> MRGSHHHHHHENLYFQGSLAVAEPVVNAADAKGTNVNDKVTASDFKLEKTAFDPNQSGNTFMAANFKVTGQVKSGDYFTAKLPDSVTGNGDVDYSNSNNTMPIADIKSTNGDVVAKATYDILTKTYTFVFTDYVNDKENINGQFSLPLFTDRAKAPKSGTYDANINIADEMFDNKITYNYSSPIAGIDKP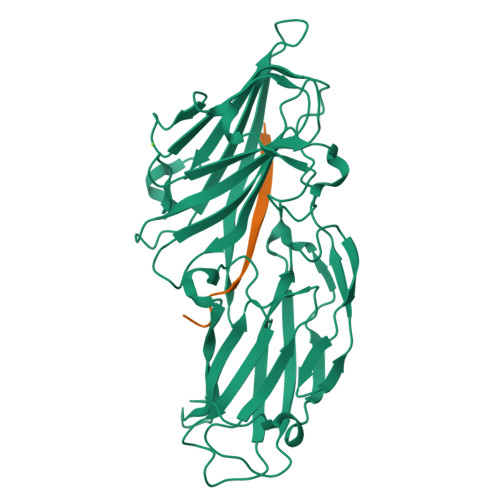NGANISSQIIGVDTASGQNTYKQTVFVNPKQRVLGNTWVYIKGYQDKIEESSGKVSATDTKLRIFEVNDTSKLSDSYYADPNDSNLKEVTGEFKDKISYKYDNVASINFGDINKTYVVLVEGHYDNTGKNLKTQVIQENIDPATGKDYSIFGWNNENVVRYGGGSADGDSAVN;> YGGGSSGGGSSGGG>MDAATTRVGLTDLTFRLLRESFADAVSWVAKNLPARPAVPVLSGVLLTGSDNGLTISGFDYEVSAEAQVGAEIVSPGSVLVSGRLLSDITRALPNKPVDVHVEGNRVALTCGNARFSLPTMPVEDYPTLPTLPEETGLLPAELFAEAISQVAIAAGRDDTLPMLTGIRVEILGETVVLAATDRFRLAVRELKWSASSPDIEAAVLV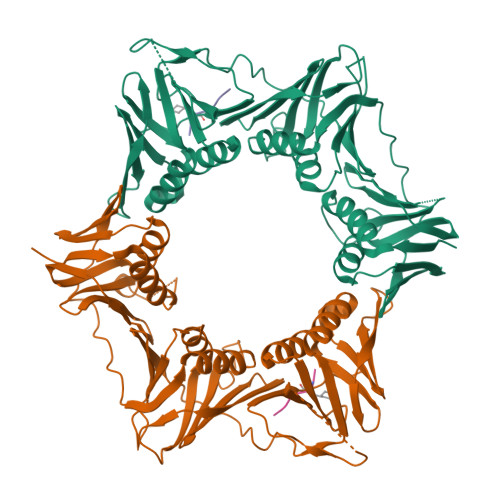PAKTLAEAAKAGIGGSDVRLSLGTGPGVGKDGLLGISGNGKRSTTRLLDAEFPKFRQLLPTEHTAVATMDVAELIEAIKLVALVADRGAQVRMEFADGSVRLSAGADDVGRAEEDLVVDYAGEPLTIAFNPTYLTDGLSSLRSERVSFGFTTAGKPALLRPVSGDDRPVAGLNGNGPFPAVSTDYVYLLMPVRLPG[4x];>XQADLF[4x]> SNAETNEITIGI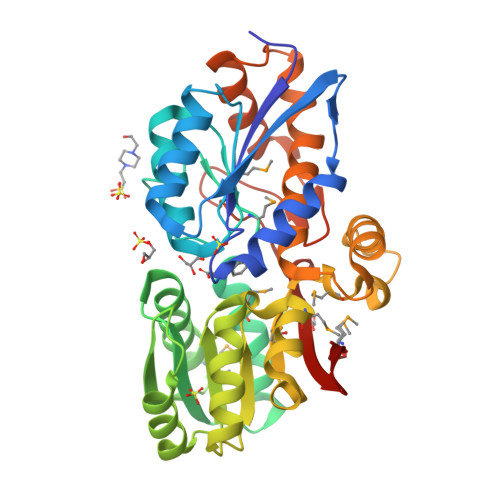TVTTTGPAAALGIPERNALEFVAKEIGGHPLKVIVLDDGGDPTAATTNARRFVTESKADVIMGSSVTPPTVAVSNVANEAQVPHIALAPLPITPERAKWSVAMPQPIPIMGKVLYEHMKKNNIKTVGYIGYSDSYGDLWFNDLKKQGEAMGLKIVAEERFARPDTSVAGQVLKLVAANPDAILVGASGTAAALPQTSLRERGYKGLIYQTHGAASMDFIRIAGKSAEGVLMASGPVMDPEGQDDSALTKKPGLELNTAYEAKYGPNSRSQFAAHSFDAFKVLERVVPVALKTAKPGTQEFREAIRKALVSEKDIAASQGVYSFTETDRYGLDDRSRILLTVKDGKYVMVK>[2x]MMPVFHTRTIESILEPVAQQISHLVIMHEEGEVDG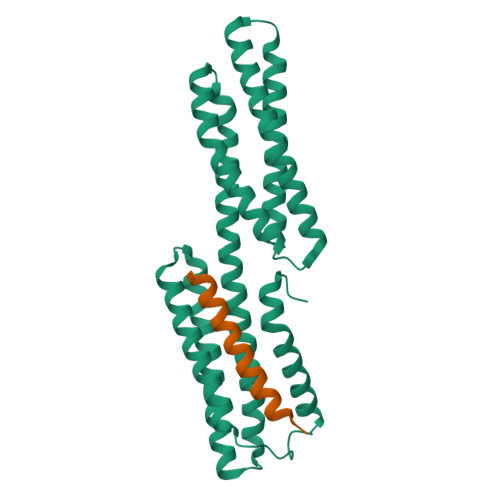KAIPDLTAPVAAVQAAVSNLVRVGKETVQTTEDQILKRDMPPAFIKVENACTKLVQAAQMLQSDPYSVPARDYLIDGSRGILSGTSDLLLTFDEAEVRKIIRVCKGILEYLTVAEVVETMEDLVTYTKNLGPGMTKMAKMIDERQQELTHQEHRVMLVNSMNTVKELLPVLISAMKIFVTTKNSKNQGIEEALKNRNFTVEKMSAEINEIIRVLQLTS;>GPLGSASARTANPTAKRQFVQSAKEVANSTANLVKTIKAL[2x]>[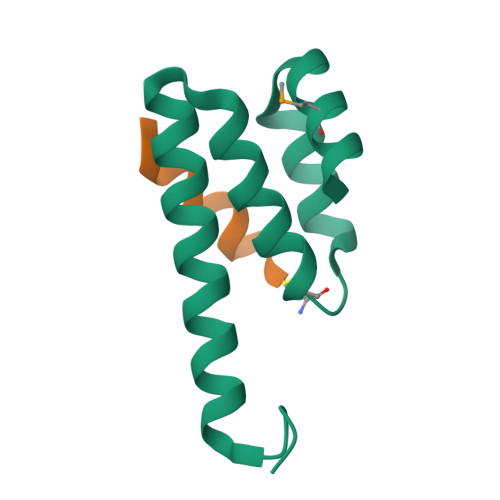2x]GPLGSDLKDAEAVQKFFLEEIQLGEELLAQGDYEKGVDHLTNAIAVCGQPQQLLQVLQQTLPPPVFQMLLTKL;>[2x]GPRLSRLLSAAGC Among five paralogues of l,d-transpeptidase in Mtb, two functional l,d-­transpeptidases, LdtMt1 (Rv0116c; 251 amino acids) and LdtMt2 (Rv2518c; MT2594; 408 amino acids), have been shown to generate 3→3 cross-links connecting two meso-diaminopimelic acid (meso-DAP) residues at the third position of the stem peptides in vitro. Here, we report the crystal structure of an N-terminally truncated Mtb LdtMt2 (LdtMt2Δ130) that encompasses residues Leu131–Ala408. In this structure, the catalytic l,d-transpeptidase domain (residues Asp251–Val378) is preceded by a bacterial immunoglobulin-like (Ig-like) Big_5 domain (residues His150–Gly250) and followed by an extended C-­terminal tail (residues Asn379–Ala408) that interacts with both domains. Cys354, His336 and Ser337 form the catalytic triad in the active site of the l,d-transpeptidase domain.

To provide a detailed structural view of how meropenem inhibits LdtMt2, we have determined the crystal structure of LdtMt2Δ130 as a covalent complex with meropenem. Each chain of the meropenem complex contains one meropenem linked to Cys354 by a thioester bond. In the meropenem-complexed structure meropenem is covalently bound to Cys354, mimicking the acyl-enzyme intermediate, and the carbonyl O atom of the opened β-lactam ring is stabilized by the oxyanion hole. In chain B of the meropenem-complex model, clear electron density for meropenem that is contiguous with the Sγ atom of Cys354 was observed, but the electron density was missing beyond the thioether S atom of meropenem. The bond distance between Cys354 Sγ and the carbonyl C atom of meropenem is 1.94 Å, which falls within the typical bond distances (1.81–2.55 Å) of carbon–sulfur single bonds. The ζ-­hydroxyl group of Tyr308 interacts with the meropenem N1 atom and the thioether S atom of meropenem C3. In addition, the pyrroline ring of meropenem is stabilized by the aromatic ring of Tyr308 through hydrophobic interactions. The backbone carbonyl groups of Ser331 and His352, as well as the side chain of His352, also make hydrogen bonds to the bound meropenem. Upon the acylation of LdtMt2 by meropenem, the active-site lid undergoes a large conformational change and partially covers the catalytic Cys354 so that the bound meropenem is accessible to the bulk solvent via three narrow paths. A large conformational change in the active-site lid of LdtMt2 upon acylation by meropenem to partially cover the bound meropenem may explain the long-lived acylated enzyme intermediate.

>MLGLGGAATRQLTFQTSSPAHLTMPYVMPGDGEVVGVGEPVAIRFDENIADRGAAEKAIKITTNPPVEGAFYWLNNREVRWRPEHFWKPGTAVDVAVNTYGVDLGEGMFGEDNVQTHFTIGDEVIATADDNTKILTVRVNGEVVKSMPTSMGKDSTPTANGIYIVGSRYKHIIMDSSTYGVPVNSPNGYRTDVDWATQISYSGVFVHSAPWSVGAQGHTNTSHGCLNVSPSNAQWFYDHVKRGDIVEVVNTVGGTLPGIDGLGDWNIPWDQWRAGNAKALEHHHHHH[2x]> MATQKETTRKRDKSVNFRLGLRNMLAQIHPDISVQTEALSELSNIAVFLGKKISHGAVTLLPEGTKTIKSSAVLLAAGDLYGKDL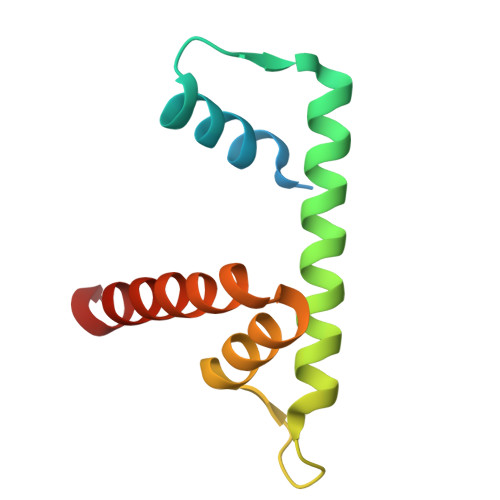GRHAVGEMTKAVTRYGSAK> MRILAIDTATEACSVALWNNGTINAHFE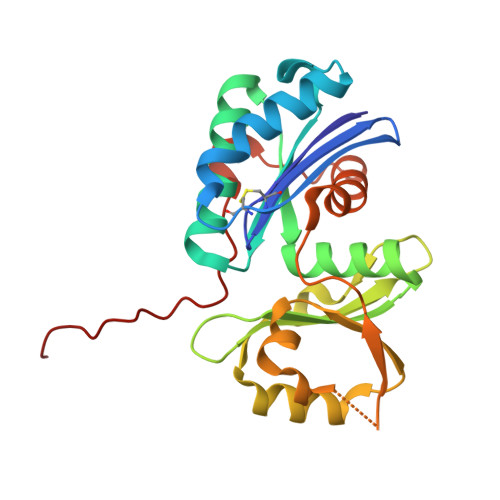LCPREHTQRILPMVQEILAASGASLNEIDALAFGRGPGSFTGVRIGIGIAQGLALGANLPMIGVSTLATMAQGAWRKTGATRVLAAIDARMGEVYWAEYQRDAQGVWQGEETEAVLKPERVGERLKQLSGEWATVGTGWSAWPDLAKECGLTLHDGEVSLPAAEDMLPIASQKLAAGETVAVEHAEPVYLRNEVAWKKLPG beta-D-glucopyranuronic acid 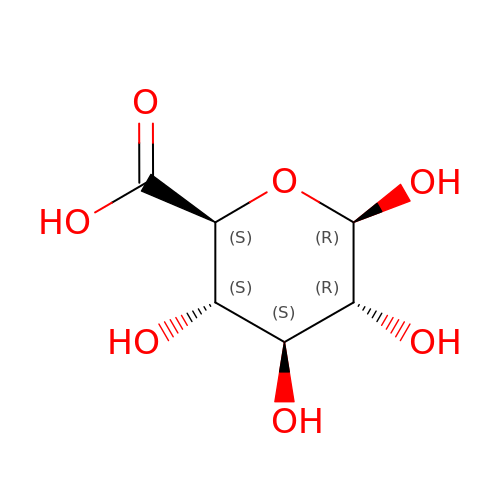| C6 H10 O7 | AEMOLEFTQBMNLQ-QIUUJYRFSA-N>[5x]AGQLSSFFRNSEQPTKPLQVVIAGAGLAGLSTAKYLADAGHKPILLEARDVLGGKIAAWKDEDGDWYETGLHIFFGAYPNIQNLFGELGINDRLQWKEHSMIFAMPNKPGEFSRFDFPETLPAPLNGI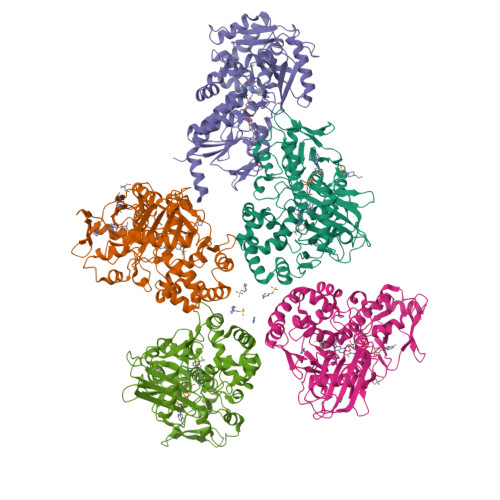WAILRNNEMLTWPEKVKFALGLLPAMVGGQAYVEAQDGFTVSEWMKKQGVPDRVNDEVFIAMSKALNFINPDELSMQCILIALNRFLQEKHGSKMAFLDGNPPERLCMPIVDHVRSLGGEVRLNSRIQKIELNPDGTVKHFALTDGTQITGDAYVFATPVDILKLLVPQEWKEISYFKKLEKLVGVPVINVHIWFDRKLKNTYDHLLFSRSSLLSVYADMSVTCKEYYDPNRSMLELVFAPAEEWVGRSDTEIIEATMQELAKLFPDEIAADQSKAKILKYHVVKTPRSVYKTIPDCEPCRPLQRSPIEGFYLAGDYTKQKYLASMEGAVLSGKLCAQSVVEDYKMLSRRSLKSLQSEVPVASHHHHHH> GSHMSRVQLALRVPDLEASIGFYSKLFGTGPAKVRPGYAN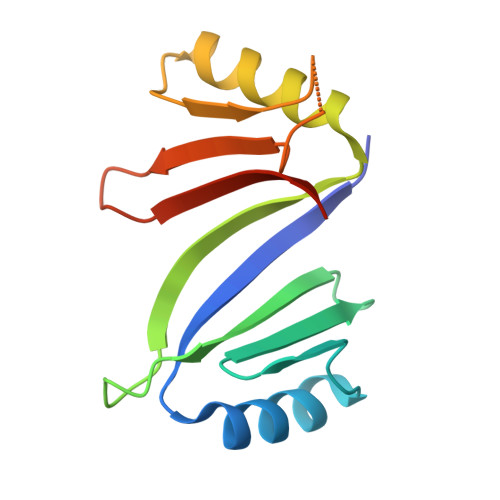FAIAEPPLKLVLIEGAGEDATRLDHLGVEVEDSAQVGHAARRLKESGLATVEENDTACCHAFQDKVWVTGPGGEPWEVYVVKGDAD The transcriptional regulator CprK from Desulfitobacterium spp. induces expression of halorespiratory genes upon binding of o-chlorophenol ligands and is reversibly inactivated by oxygen through disulphide bond formation. The CprK associated with the o-chlorophenolacetic acid (OCPA) reductive dehalogenase (CprAB) from D. dehalogenans and the closely related D. hafniense has been shown to bind OCPA with μM affinity leading to sequence-specific DNA-binding, and ultimately transcriptional activation of the associated cpr gene cluster (Pop et al., 2004; 2006; Gabor et al., 2006; Joyce et al., 2006; Mazon et al., 2007). Members of this family are homodimeric and contain an N-terminal sensor domain linked via a long α-helix (involved in formation of the dimer interface) to the C-terminal helix–turn–helix (HTH) DNA-binding domain. We here present crystal structures of the oxidized ligand-free (3.2 Å) and reduced ligand-free (2.0 Å), OCPA-bound (1.8 Å) and DNA-bound (1.8 Å) D. hafniense CprK in addition to an intermediate OCPA-bound structure obtained by soaking ligand-free crystals (2.0 Å).

Crystals of the ligand-free CprKC200S can be soaked with high concentrations of o-halogenated phenol acetic acid ligands without any apparent detrimental effects. The corresponding structures reveal that OCPA is bound in both sensor domains and establishes a near identical network of polar and hydrophobic interactions within the active site as described for the cocrystallized structures. A significant structural rearrangement of both sensor domains similar to that observed when comparing ligand-free and OCPA-bound CprKC200S structures has occurred, but in absence of significant DNA-binding domain reorientation. While the conformation of the central α-helices (Ser-108 to Ala-142) has become identical to the OCPA cocrystallized structures, the sensor domain β-barrels have only partly rotated along the Ser-108 hinge points. This is likely due to the fact that full rotation as is observed for the OCPA-bound structures would lead to minor clashes with crystal symmetry related neighbouring molecules for both monomers. While the N-terminal residue Phe-20 has effectively replaced the previous position of Phe-19 in both monomers, as occurs during conversion from the ligand-free to the ligand cocrystallized structure, the preceding N-terminal residues remain unstructured in both monomers. We therefore speculate that reorganization of the N-terminus only occurs during or following DNA-binding domain reorientation. Furthermore, in view of the similar resolution and near identical crystal packing, a direct B-factor comparison is feasible between the ligand-free CprKC200S and corresponding OCPA-soaked structure. This reveals that ligand binding leads to significantly decreased B-factors for both β-barrels as well as the C-terminal section of the central α-helices (average decrease of ∼6 Å2).

>[2x]MSVEGLGKDFCGAIIPDNFFPIEKLRNYTQMGLIRDFAKGSAVIMPGEEITSMIFLVEGKIKLDIIFEDGSEKLLYYAGGNSLIGKLYPTGNNIYATAMEPTRTCWFSEKSLRTVFRTDEDMIFEIFKNYLTKVAYYARQVAEMNTYNPTIRILRLFYELCSSQGKRVGDTYEITMPLSQKSIGEITGVHHVTVSRVLASLKRENILDKKKNKIIVYNLGELKHLSEQTSYYSDPNSSSVDKLAAALDHH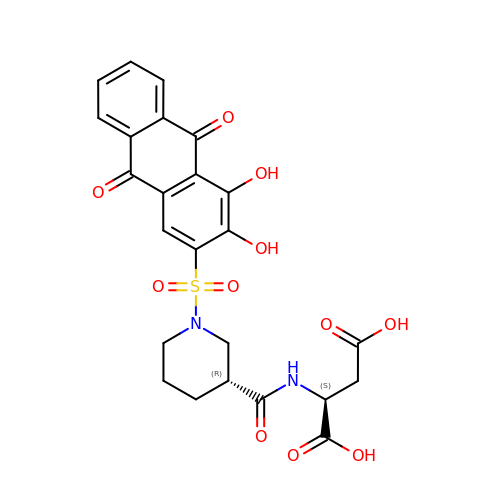N-[(3R)-1-(3,4-dihydroxy-9,10-dioxo-9,10-dihydroanthracene-2-sulfonyl)piperidine-3-carbonyl]-L-aspartic acid | C24 H22 N2 O11 S | HWQZQOYBMBRIAX-ABAIWWIYSA-N> GSHHVVPNEVVVQRLFQVKGRRVVRATEVPVSWESFKNGDCFILDLGNNIHQWCGSNSNRYERLKATQVSKGIRDNERSGRARVHVSEEGTE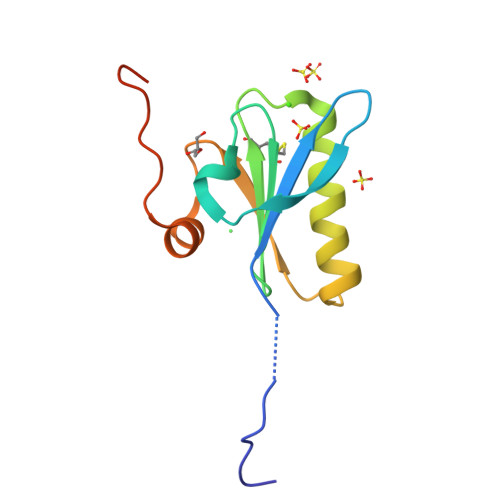PEAMLQVLGPKPALPAGTEDTAKEDAA> SLRREMQEILPGLFLGPYSSAMKSKLPVLQKHGITHIICIRQNIEANFIKPNFQQLFRYLVLDIADNPVENIIRFFPMTKEFIDGSLQMGGKVLVHGNAG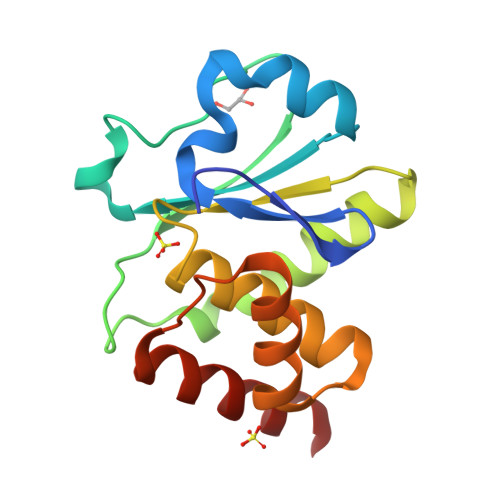ISRSAAFVIAYIMETFGMKYRDAFAYVQERRFCINPNAGFVHQLQEYEAIYLAK> LPAQVAFTPYAPEPGSTCRLREYYDQTAQMCCSKCSPGQHAKVFCTKTSDTVCDSCEDSTYTQLWNWVPECLSCGSRCSSDQVETQACTREQNRICTCRPGWYCALSKQEGCRLCAPLRKCRPGFGVARPGTETSDVVCKPCAPGTFSNTTS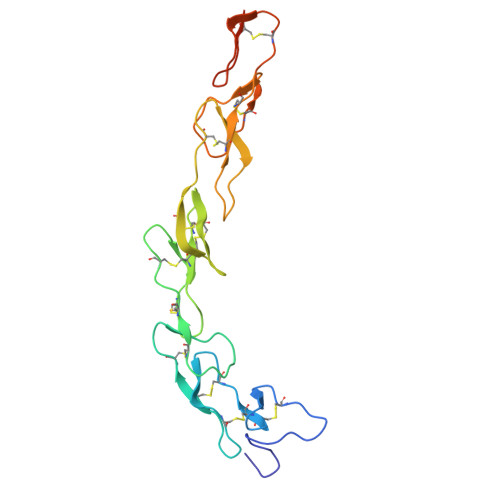STDICRPHQICNVVAIPGNASMDAVCTSTSPTRSMAPG> ACTKNAIAQTGFNKDKYFNGDVWYVTDYLNLEPDDVPKRYCAALAAGTASGKLKEALYHYDPKTQDTFYDVSELQVESLGKYTANFKKVDKNGNVKVAVTAGNYYTFTVMYADDSSALIHTC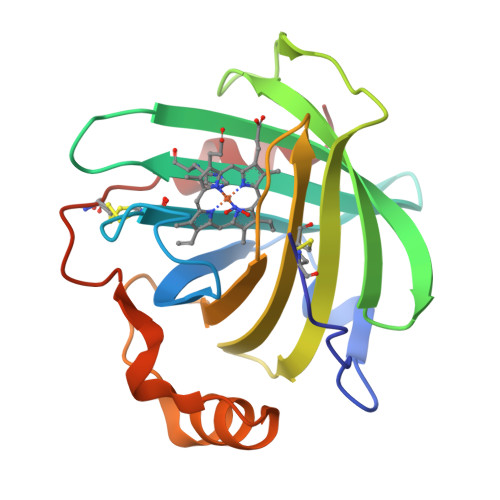LHKGNKDLGDLYAVLNRNKDAAAGDKVKSAVSAATLEFSKFISTKENNCAYDNDSLKSLLTK> MKLSPREIEKLGLHNAGYLAQKRLARGLRLNYTEAVALIATQIMEFVRDGDKTVAQLMSIGRELLGRRQVLPAVPKLVESVQVEATFPDGTELVTIHDPIACENGNLELALLGSFLPVPSLDKFTANDEDNRIPGEIIVVGGNLVLNDGRKAVILKVVNNGDRPVQVGSHYHFIELNPYLTFDRRKAYGMRLNIAAGNASRFEPGEMKEVLLVSIGGNKVIRGGNAIADGPVNASNCIAAMQAVITRGFGHVEEANAAEGQTGEDASCPFTTVISREEYANKYGPTTGDKIRLGDTALFAEIEKDFAIYGDECTFGGGKVIRDGMGQSCGHPPALSLDTVITNAVIIDYSGIIKADIGIKDGLIHSIGKSGNPDVMDGVFQNMTTGVNTEVIAGEGLIVTAGAIDCHVHYICPQLVYEAVTSGITTLVGGGTGPTAGTRATTCTPAPIQMKLMLQSTDDLPLNFGFTGKGNCAKPDELHEIIKAGAMGLKLHEDWGTTPAAIDSCLTIAEQYDIQVNIHTDTLNESGFV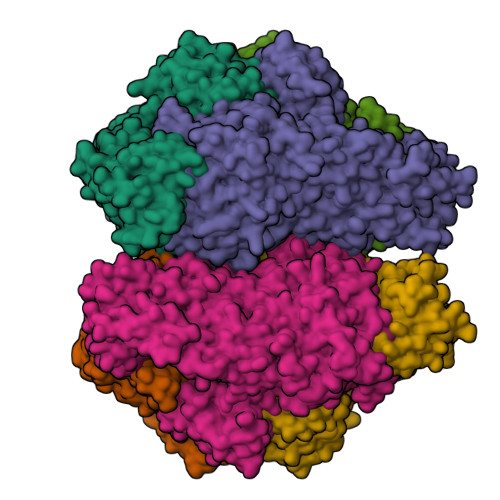EHTIAAFKGRTIHTYHSEGAGGGHAPDIIKVCGEKNVLPSSTNPTRPLTSNTIDEHVDMLMVCHHLDANIAEDVAFSASRIREATIAAEDILHDMGAISIISSDSQAMGRIGEVISRTWQTADKMKSARGPLQPGEEANDNFRIKRYVAKYTINPAIANGFSQYVGSVEVGKLADLVMWKPSFFGAKPEMVIKGGEVAYANMGDPNASIPTPEPVKMRPMYGALGKAGGALSIAFVSKAALDQRVKVLYGLNKRVEAVSNVRKLTKLDMKLNDALPAITVDPDSYTVTADGVVLTCFVATTVPLSRNYFIF;> MKLSPREIEKLGLHNAGYLAQKRLARGLRLNYTEAVALIATQIMEFVRDGDKTVAQLMSIGRELLGRRQVLPAVPKLVESVQVEATFPDGTELVTIHDPIACENGNLELALLGSFLPVPSLDKFTANDEDNRIPGEIIVVGGNLVLNDGRKAVILKVVNNGDRPVQVGSHYHFIELNPYLTFDRRKAYGMRLNIAAGNASRFEPGECKEVLLVSIGGNKVIRGGNAIADGPVNASNCIAAMQAVITRGFGHVEEANAAEGQTGEDASCPFTTVISREEYANKYGPTTGDKIRLGDTALFAEIEKDFAIYGDECTFGGGKVIRDGMGQSCGHPPALSLDTVITNAVIIDYSGIIKADIGIKDGLIHSIGKSGNPDVMDGVFQNMTTGVNTEVIAGEGLIVTAGAIDCHVHYICPQLVYEAVTSGITTLVGGGTGPTAGTRATTCTPAPIQMKLMLQSTDDLPLNFGFTGKGNCAKPDELHEIIKAGAMGLKLHEDWGTTPAAIDSCLTIAEQYDIQVNIHTDTLNESGFVEHTIAAFKGRTIHTYHSEGAGGGHAPDIIKVCGEKNVLPSSTNPTRPLTSNTIDEHVDMLMVCHHLDANIAEDVAFSASRIREATIAAEDILHDMGAISIISSDSQAMGRIGEVISRTWQTADKMKSARGPLQPGEEANDNFRIKRYVAKYTINPAIANGFSQYVGSVEVGKLADLVMWKPSFFGAKPEMVIKGGEVAYANMGDPNASIPTPEPVKMRPMYGALGKAGGALSIAFVSKAALDQRVKVLYGLNKRVEAVSNVRKLTKLDMKLNDALPAITVDPDSYTVTADGVVLTCFVATTVPLSRNYFIF> NFVLPELPSVPDTLPTASAGASTSASEDIDFDDLSRRFEELKK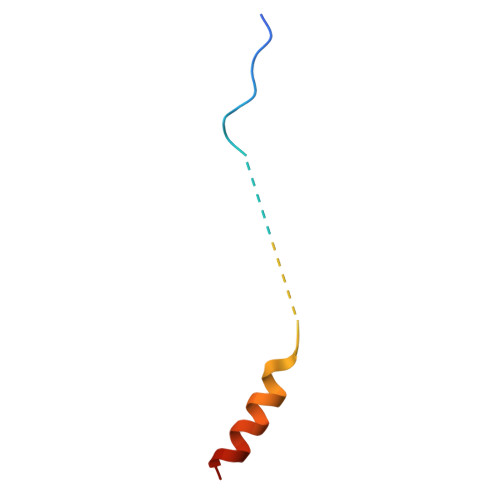KT>[5x]SGSVSKWVRLNV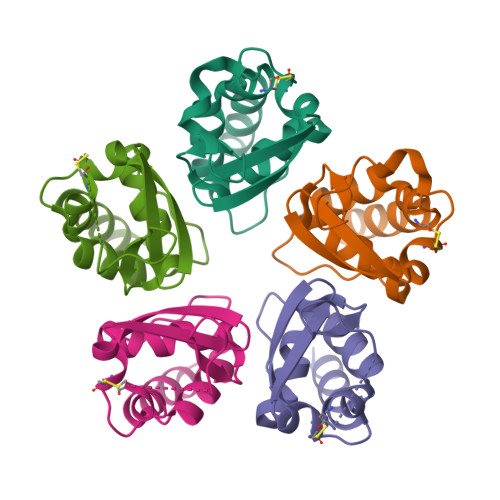GGTYFLTTRQTLCRDPKSFLYRLCQADPDLDSDKDETGAYLIDRDPTYFGPVLNYLRHGKLVINKDLAEEGVLEEAEFYNITSLIKLVKDKIRER> GFPTELKPGTNQFLTTDDGVSAPILPNFHPTP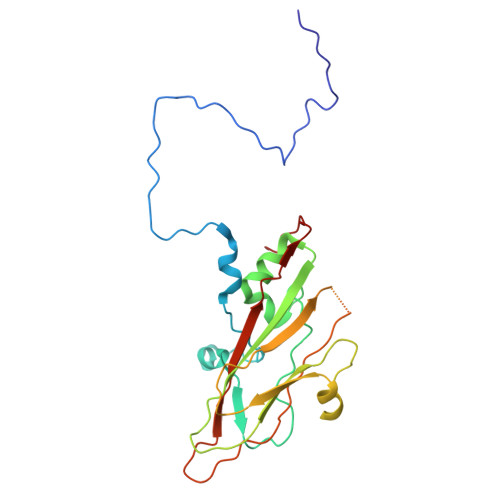CIHIPGEVRNLLELCQVETILEVNNVPTNATSLMERLRFPVSAQAGKGELCAVFRADPGRSGPWQSTLLGQLCGYYTQWSGSLEVTFMFTGSFMATGKMLIAYTPPGGPLPKDRATAMLGTHVIWDFGLQSSVTLVIPWISNTHYRAHARDGVFDYYTTGLVSIWYQTNYVVPIGAPNTAYIIALAAAQKNFTMQLCKDASDIL> MGATGDAEQPRGPSGAERGGLELGDAGAAGQLVLTNPW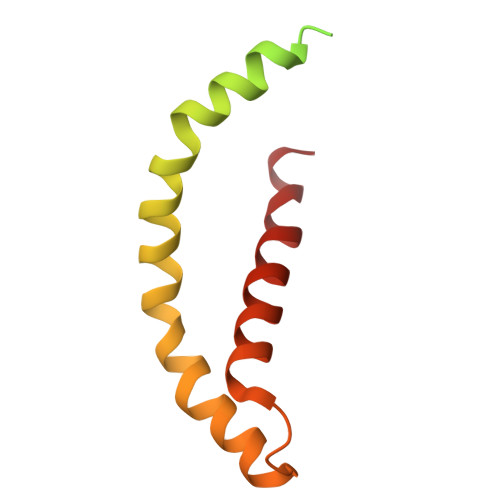NIMIKHRQVQRRGRRSQMTTSFTDPAISMDLLRAVLQPSINEEIQTVFNKYMKFFQKAALNVRDNVGEEVDAEQLIQEACRSCLEQAKLLFS>MKI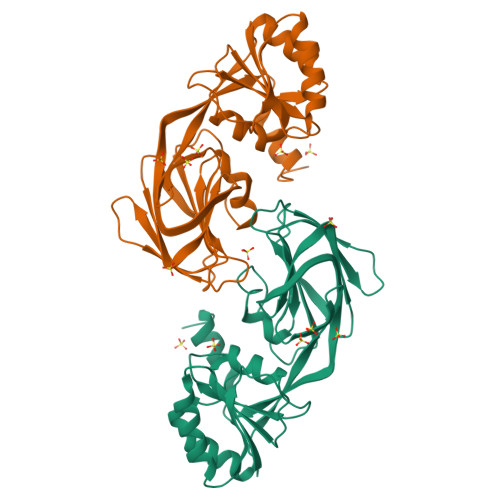AILYREEREKEGEFLKEKISKEHEVIEFGEANAPGRVTADLIVVVGGDGTVLKAAKKAADGTPMVGFKAGRLGFLTSYTLDEIDRFLEDLRNWNFREETRWFIQIESELGNHLALNDVTLERDLSGKMVEIEVEVEHHSSMWFFADGVVISTPTGSTAYSLSIGGPIIFPECEVLEISPIAPQFFLTRSVVIPSNFKVVVESQRDINMLVDGVLTGKTKRIEVKKSRRYVRILRPPEYDYVTVIRDKLGYGRRIE[4x]> PVNLNNLEAKRIVACDDPDFLTSYFAHSRLHHLSAWKANLKDKFLNENIHKYTKITDKDTYIIFHIDFDCFFATVAYLCRSSSFSACDFKRDPIVVCHGTKNSDIASCNYVARSYGIKNGMWVSQAEKMLPNGIKLISLPYTFEQFQLKSEAFYSTLKRLNIFNLILPISIDEAVCVRIIPDNIHNTNTLNARLCEEIRQEIFQGTNGCTVSIGCSDSLVLARLALKMAKPNGYNITFKSNLSEEFWSSFKLDDLPGVGHSTLSRLESTFDSPHSLNDLRKRYTLDALKASVGSKLGMKIHLALQGQDDEESLKILYDPKEVLQRKSLSIDINWGIRFKNITQVDLFIERGCQYLLEKLNEINKTTSQITLKLMRRCKDAPIEPPKYMGMGRCDSFSRSSRLGIPTNEFGIIATEMKSLYRTLGCPPMELRGLALQFNKLVDVGPDNNQLK

Rev1 is a translesion DNA synthesis (TLS) polymerase involved in the bypass of adducted-guanine bases and abasic sites during DNA replication. During damage bypass, Rev1 utilizes a protein-template mechanism of DNA synthesis, where the templating DNA base is evicted from the Rev1 active site and replaced by an arginine side chain that preferentially binds incoming dCTP. Notably, Rev1 is the only DNA polymerase known to use an amino-acid side chain to encode for an incoming nucleotide, instead of a templating DNA base. Additionally, Rev1 does not undergo large conformational changes upon incoming nucleotide binding.

To obtain structural insight for the interaction of Rev1 and an incoming dTTP, we determined a ternary complex (Rev1/DNA/dNTP) structure of Rev1 with an incoming dTTP. The Rev1/DNA binary complex crystals were then transferred to a cryoprotectant containing dTTP and CaCl2 to generate Rev1-dTTP ternary complex crystals. Importantly, Ca2+ permits incoming nucleotide binding but does not facilitate catalysis in crystallo. The resulting Rev1/DNA/dTTP ternary complex crystal diffracted to 1.70 Å and was in space group P212121. The overall structure of the Rev1-dTTP ternary complex is similar to the Rev1-dCTP ternary complex structure (RMSD = 0.228 Å), including the evicted templating guanine base, the R324 protein template, and Rev1 active site side chains. The incoming dTTP is coordinated by the R324 through a single non-planar hydrogen bond between the O2 of the Watson-Crick edge and the Nε of R324. The non-planar R324-dTTP interaction leads to a 2.6 Å movement in the dTTP base towards the primer terminal dG. To accommodate the dTTP, the primer terminal dG moves 1.4 Å downward from the conformation seen in the Rev1-dCTP ternary complex structure. This brings the 3′-OH of the primer terminal dG 4.4 Å away from Pα of the incoming dTTP, which is ~1 Å increase compared to the Rev1-dCTP ternary complex structure.>[2x]AYAYMTIDIGGGNPSVEMALNSDYEVIELTPLNDEGQKVVNDIDDWEKTDFKKVIDDIITDCSEHGYVKKSKEILISTVYENTEDNTYKKAVKKQLNDVTEKYKTTYRMESLESDMQTR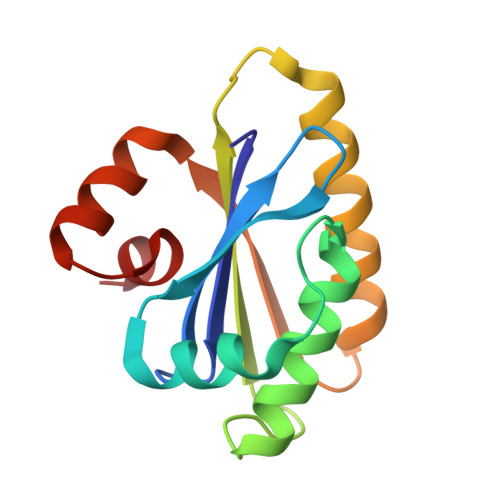EKAKKEGVSTGSYIKS> MPLPNAVVQGYTSVRGPKRPLDHFYGRTPLNIDTLWHWVKFPHRYDNLRFAVCFWAFLVSAHFANKKQRNLRVEWEKNMEIQKKLHPSGLWSEEQAFAAAEKLGRPKAGHP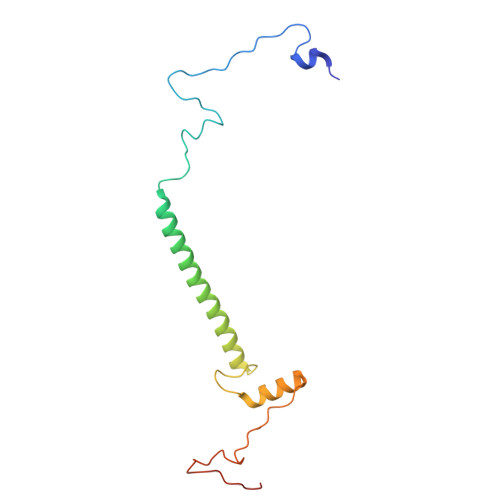MRVFEDGYQQFDLKPKLFDPDEEAHH>[2x]GHMAIAPNTRVLVAGYGLPAEFCVTTLIGMGVEIDKIAVATHREDNRNSGLHSMLRLRNIQFTTAAANSEEFYEFGANFAPDMIISMHYRSLIPGRFLKLAKKGSVNLHPSLLPAYRGTNSVAWVIINGESETGFSYHRMDENFDTGAILLQERISVEETDTAFSLFHRQIARAMLRLEEVILKLDQGDPGFAQLGEASYYARELPFGGVIDPRWSEVQIDRFIRAMFFPPFPPAVLKIDGKVY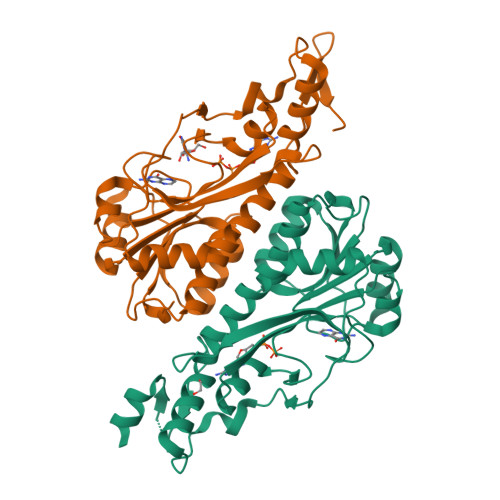YVPSIDIYRSLMRGIPS> GDIVSEKKPATEVDPTHFEKRFLKRIRDLGEGHFGKVELCRYDPEGDNTGEQVAVKSLKPESGGNHIADLKKEIEILRNLYHENIVKYKGICTEDGGNGIKLIMEFLPSGSLKEYLPKNKNKINLKQQLKYAVQICKGMDYLGSRQYVHRDLAARNVLVESEHQVKIGDFGLTKAIETDKEYYTVKDDRDSPVFWYAPECLMQSKFYIASDVWSFGVTLHELLTYCDSDSSPMALFLKMIGPTHGQMTVTRLVNTLKEGKRLPCPPNCPDEVYQLMRKCWEFQPSNRTSFQNLIEG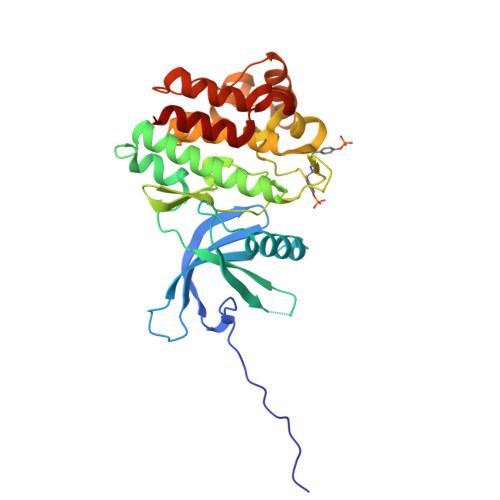FEALLK>[4x]RPHKCHLCGRAFRTVTLLRNHLNTHTGTRPHKCPDCDMAFVTSGELVRHRRYKHTHEKPFKCSMCDYASVEVSKLKRHIRSHTGERPFQCSLCSYASRDTYKLKRHMRTHSGEKPY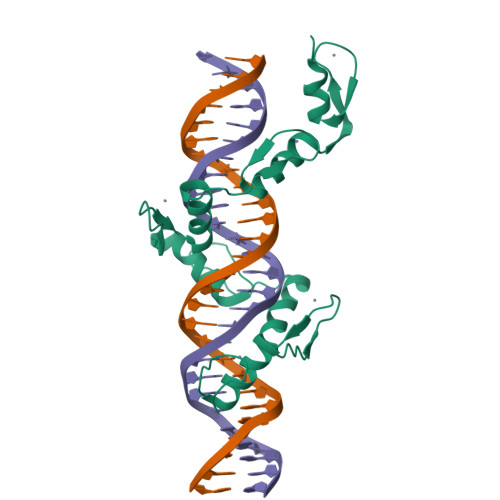ECYICHARFTQSGTMKMHILQKHTENVAKFHCPHCDTVIARKSDLGVHLRKQHSYIEQGKKCRYCDAVFHERYALIQHQKSHK> VVTYNTLIDGLAKAGRLEEALQLFQEMKEKGVKPSVVTYNTLID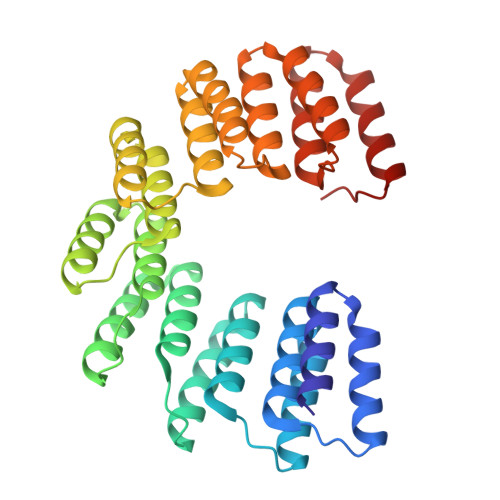GLAKAGRLEEALQLFQEMKEKGVKPSVVTYNTLIDGLAKAGRLEEALQLFQEMKEKGVKPSVVTYNTLIDGLAKAGRLEEALQLFQEMKEKGVKPSVVTYNTLIDGLAKAGRLEEALQLFEEMKEKGVKPSVVTYNTLIDGLAKAGRLEEALQLFQEMKEKGVKPSVVTYNTLIDGLAKAGRLEEALQLFEEMKEKGVKPSVVTYNTLIDGLAKAGRLEEALQLFEEMKEKGVKPSVVTYNTLIDGLAKAGRLEEALQLFQEMKEKGVKPS>MVLYFIGLGLYDERDITVKGLEIAKKCDYVFAEFYTSLMAGTTLGRIQKLIGKEIRVLSREDVELNFENIVLPLAKENDVAFLTPGDPLVATT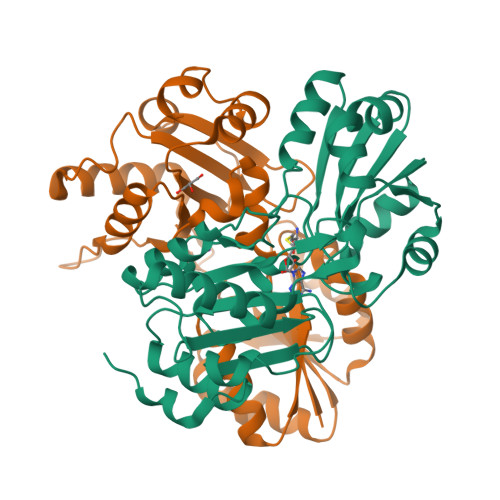HAELRIRAKRAGVESYVIHAPSIYSAVGITGLHIYKFGKSATVAYPEGNWFPTSYYDVIKENAERGLHTLLFLDIKAEKRMYMTANEAMELLLKVEDMKKGGVFTDDTLVVVLARAGSLNPTIRAGYVKDLIREDFGDPPHILIVPGKLHIVEAEYLVEIAGAPREILHVNV[2x]Cas13d is a class 2 type VI-D CRISPR-Cas RNA-guided RNase. Cas13 family is the only family of class 2 Cas enzymes known to exclusively target single-stranded RNA. Analogously to the other members of the Cas13 superfamily, Cas13d also contains two R-X4-H HEPN motifs, but bears little overall similarity to the amino acid sequences of Cas13a and Cas13b. Owing to its biochemical properties, especially small size, lack of constraints on the target flanking sequences, and highly efficient and specific target RNA cleavage, Cas13d is a promising candidate for RNA engineering and editing.

The binary complex was obtained by the selenomethionine (SeMet)-derived UrCas13d (R288A/R823A) mutant co-expressed with CRISPR RNA in vivo. The SeMet-labeled structure was subsequently used as a model to solve the crystal structure of the unlabeled UrCas13d (R288A/R823A) binary complex at 1.86 Å resolution using the molecular replacement method. A mature 50-nt crRNA was determined in the binary complex. It originated from an in vivo transcript encoded by a co-expressed CRISPR template, which was further processed by UrCas13d itself in E. coli cells. The crRNA consists of a 30-nt repeat region (C(-30)-C(-1)) and 20-nt spacer region (U(1)-A(20)). The high resolution of the binary complex unambiguously shows an octahedral-shaped electron density around the phosphate group of the nucleotide C(-7). Considering that Mg2+ and Na+ are metal ions provided in buffer systems during the purification and crystallization, a penta-hydrated Mg2+ was built into the present structure. Moreover, the (Mg(H2O)5)2+ ion forms hydrogen bonds with the phosphate groups of the nucleotides A(-5), A(-3), and A(-2), as well as the side chain of residue D178. In addition, a tetra-hydrated Mg2+ was found to coordinate with two backbone oxygen atoms of residues R137 and E140 from a loop region of NTD.

> MAKKNKMKPRELREAQKKARQLKAAEINNNAAPAIAAMPAAEVIAPVAEKKKSSVKAAGMKSILVSENKMYITSFGKGNSAVLEYEVDNNDYNKTQLSSKDNSNIELGDVNEVNITFSSKHGFGSGVEINTSNPTHRSGESSPVRGDMLGLKSELEKRFFGKTFDDNIHIQLIYNILDIEKILAVYVTNIVYALNNMLGIKDSESYDDFMGYLSARNTYEVFTHPDKSNLSDKVKGNIKKSLSKFNDLLKTKRLGYFGLEEPKTKDTRASEAYKKRVYHMLAIVGQIAQCVFHDKSGAKRFDLYSFINNIDPEYRDTLDYLVEERLKSINKDFIEGNKVNISLLIDMMKGYEADDIIRLYYDFIVLKSQKNLGFSIKKLREKMLEEYGFRFKDKQYDSVRSKMYKLMDFLLFCNYYRNDVAAGEALVRKLRFSMTDDEKEGIYADEAAKLWGKFRNDFENIADHMNGDVIKELGKADMDFDEKILDSEKKNASDLLYFSKMIYMLTYFLDGKEINDLLTTLISKFDNIKEFLKIMKSSAVDVECELTAGYKLFNDSQRITNELFIVKNIASMRKPAASAKLTMFRDALTILGIDDNITDDRISEILKLKEKGKGIHGLRNFITNNVIESSRFVYLIKYANAQKIREVAKNEKVVMFVLGGIPDTQIERYYKSCVEFPDMNSSLEAKRSELARMIKNISFDDFKNVKQQAKGRENVAKERAKAVIGLYLTVMYLLVKNLVNVNARYVIAIHCLERDFGLYKEIIPELASKNLKNDYRILSQTLCELCDDRNESSNLFLKKNKRLRKCVEVDINNADSSMTRKYANCIAHLTVVRELKEYIGDIRTVDSYFSIYHYVMQRCITKRGDDTKQEEKIKYEDDLLKNHGYTKDFVKALNSPFGYNIPRFKNLSIEQLFDRNEYLTEKLEHHHHHH>SNAMKILTVNVHAWLEENQMEKIDILARTIAEKQYDVIAMQEVNQLMNNKIIFDDIREENYAWVLLETLQKYTDTDYYLHWSNSHIGFGKYNEGVAVITRHKIKAEDEFYCTFAQSVRTISARRIVSITINYEGQDIEFYSCHMNLPNCETEDMGKNIQTILNRTQNSNLKILMGDFNTDAIGNVAAYENILSQGLFDTYVMAEKKDDGITVDKSIHGWDNDKAKKRLDYIFSNKELKVKESKVIFNNKNKEIVSDHFGIE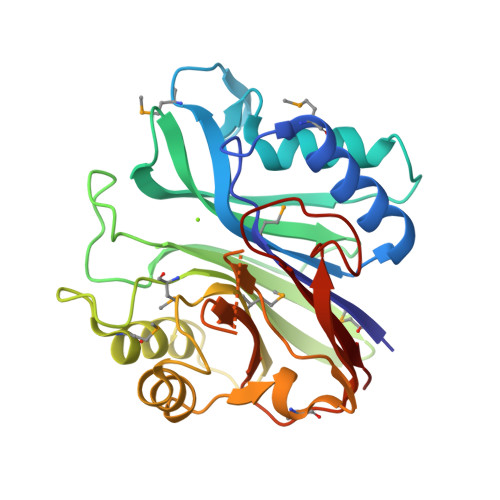VKIEF[2x]>[2x]MDVVRASRNAKVKGKFRESYLSPAQSVKPKINTEEKLPREKLNPPTPSIYLESKRDAFSPVLLQFCTDPRNPITVIRGLAGSLRLNLGLFSTKTLVEASGEHTVEVRTQVQQPSDENWDLTGTRQIWPCESSRSHTTIAKYAQYQASSFQESLQEEKESEDEESEEPDSTTGTPPSSAPDPKNHHIIKFGTNIDLSDAKRWKPQLQELLKLPAFMRVTSTGNMLSHVGHTILGMNTVQLYMKVPGSRTPGHQENNNFCSVNINIGPGDCEWFAVHEHYWETISAFCDRHGVDYLTGSWWPILDDLYASNIPVYRFVQRPGDLVWINAGTVHWVQATGWCNNIAWNVGPLTAYQYQLALERYEWNEVKNVKSIVPMIHVSWNVARTVKISDPDL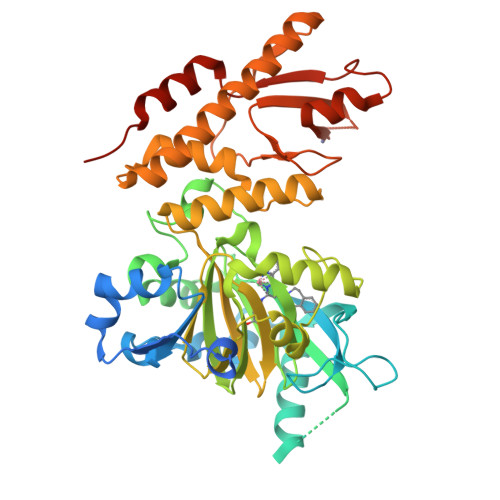FKMIKFCLLQSMKHCQVQRESLVRAGKKIAYQGRVKDEPAYYCNECDVEVFNILFVTSENGSRNTYLVHCEGCARRRSAGLQGVVVLEQYRTEELAQAYDAFTLAPASTSRHHHHHH The double-stranded (ds)RNA virus Giardia lamblia virus (GLV or Giardiavirus) exclusively infects G. duodenalis. ORF1 expresses a capsid protein (CP) that assembles an icosahedral capsid. The GLV capsid comprises 60 copies of CP dimers named subunits A and B (CP-A and CP-B) in the triangulation number (T) = 1 icosahedral asymmetric unit. The overall structure of the GLV CP shows a typical α-helix-rich α+β fold commonly adopted in the Totiviridae and other icosahedral dsRNA viruses.

The first high-resolution capsid structure of two GLV subtypes was determined using cryogenic electron microscopy (cryo-EM) single-particle analysis at a resolution of 2.1 Å and 2.6 Å for GLV-HP and GLV-CAT, respectively. GLV-HP tends to form aggregates and accumulate below the trophozoite plasma membrane and inside the cell body, whereas GLV-CAT does not form aggregates, is scattered in the trophozoite, and does not accumulate in the cell body. Hence, this C-terminal interlocking is identified in two directions in the GLV-CAT capsid: CP-A to CP-B and CP-B to CP-A. The C-terminal interlocking includes the same amino acid pairs as Arg671–Asp922 and Lys774–Asp927; however, more intersubunit interactions are identified in GLV-CAT. In the CP-A to CP-B direction, only two possible hydrogen bonds—Arg675–Asp928 and E872–N917—are present in GLV-CAT. In the C-terminal extension of the GLV-CAT subunits, similar swapping occurs structurally on the Lys902 residue. Notably, Phe320 in GLV-HP forms intrasubunit interactions with Val184, Leu590, and Asn592 in the CP-B; however, in GLV-CAT, the corresponding Leu320 in CP-B interacts with Asn112 and Gln282 residues in the adjacent CP-A. The switching between the intrasubunit and intersubunit interactions by the F320L point mutation largely contributes to driving the observed structural change in the variable loop. The Phe320 or Leu320 residue in the CP-A is located near the 5-fold axis, which might also affect the observed structural variation there. This additional CP–CP interaction, which is mediated by Leu320 and the variable loop in GLV-CAT, should make the CPs’ network in the capsid more robust. With the more robust C-terminal interlocking in the GLV-CAT capsid, the capsid assembly of GLV-CAT is structurally distinct from that of GLV-HP.

>PENITLDTLNTQNDYEETHGESPEVPKASIAPAGRQNVPVLQQNQENKDNHALGGSEDAKDEREIRFSAIKTLYNYYSEGPSTPIMPHLVNRLRGLDALAKIDATLTKVDMNAAYIFALRPTFPYSYGYKQRFSNRRLTTSAVCYARTGLSSFLTVNKTYTSNSPLKGGSRGWPIFNVGVSPHVAEPHMRTLSPIGLEVFSQNLATFSKTLLTASSKVFTQSLYTADILSIFGEVFLPHVMQPVSNYTPILVRALLALIHILGPGSGNCSLSSSIFESSIPQFFTVSHSTNMSNRTRYCLHTWSAYKDMFRNGIPPQSTLPPTLAPEGSSARVLIPAALVTSPMFPWLLALVSSGPQFFLYSKDASINTVDIGSRGRITSPIPDVANLDLHRLWNLFRFDGHRYIDVVIVGVDRDYVWPYQNGVYVHGGKGPNGTDNYGNADVHDGIGTIFSSFNDNVNVQTSDLILGLLTLWNHITTTYATEEEVTMAIKIAAAFALVYPVQPIVYSGCPRAFQSHTSYYQPSSENCYTTDTAEVKSTWDTVELSVQVNNAMVLGMTLPFGQPTVSSAQWFNNIDKAEISMFKVGNLPLQNLDYLSLDMMEFYAPTTGQLYDIRSDNLILSAHRTVNLGIGYTALADFFAYLASVPAQSFYHDRMVTSPISKQTYSVYERFIERFVDDFVGWDRCDLFNLDTLLAAKRIAGVASSPIPWHCSLQRCPLPIIMHYTGLHFGQEHITVRDVAGVEGLQQIVMRNDQGKIVVDALGTAAPSRLAVKLDWSRLSAWYSDTTCAIPLSDRVMEIINYAAIWDPTQERRATGFVYTYFSPNFLSSFNASEPIFNTSINLTPPYDDTSHTVIQNLSMPQMLSFDPYYESTFYVVSADNEWIPTSGPAWKVPYLENVVKRSGRRLLAELRIASNNGSGDRTFLDDV[2x]>MMSIAQVRSAGSAGNFYTDKDNYYVLGSMGERWAGRGAEQLGLQGSVDKDVFTRLLEGRLPDGADLSRMQDGSNRHRPGYDLTFSAPKSVSMMAMLGGDKRLIDAHNQAVDFAVRQVEALASTRVMTDGQSETVLTGNLVMALFNHDTSRDQEPQLHTHAVVANVTQHNGEWKTLSSDKVGKTGFIENVYANQIAFGRLYREKLKEQVEALGYETEVVGKHGMWEMPGVPVEAFSGRSQTIREAVGEDASLKSRDVAA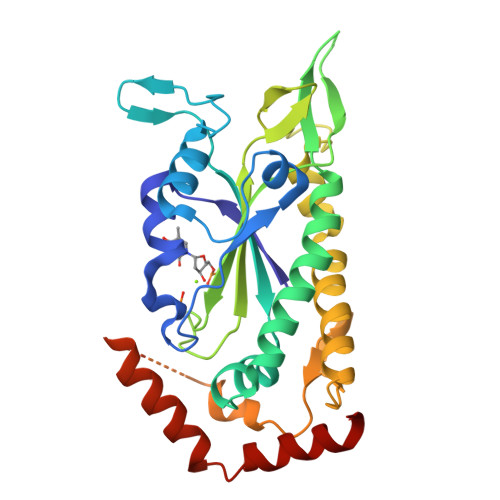LDTRKSKQHVDPEIKMAEWMQTLKETGFDIRAYRDAADQRADS[2x]>MAALRNGLEGSSEETSFHDESLQDDREEIENNSYHMHPAGIILTKVGYYT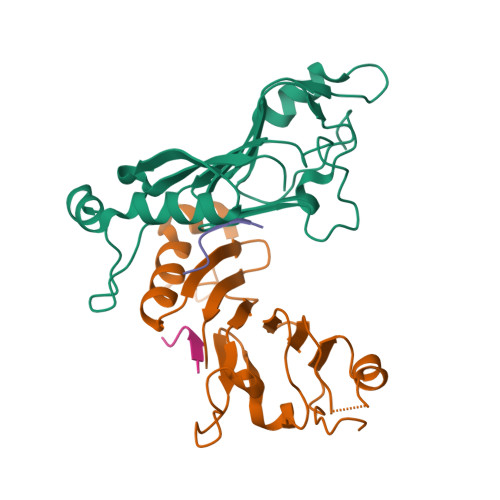IPSMDDLAKITNEKGECIVSDFTIGRKGYGSIYFEGDVNLTNLNLDDIVHIRRKEVVVYLDDNQKPPVGEGLNRKAEVTLDGVWPTDKTSRCLIKSPDRLADINYEGRLEAVSRKQGAQFKEYRPETGSWVFKVSHF[2x];>[2x]SKYGLQDSDEEEEEHPSKTSTKKLKTAPLPPASQTTPLQMALNGKPAPPPQVEKKGQLEHHHHH>MKYILVTGGVISGIGKGIIASSVGTILKSCGLHVTSIKIDPYINIDAGTFSPYEHGEVFVLDDGGEVDLDLGNYERFLDIRLTKDNNLTTGKIYQYVINKERKGDYLGKTVQVVPHITDAIQEWVMRQALIPVDEDGLEPQVCVIELGGTVGDIESMPFIEAFRQFQFKVKRENFCNIHVSLVPQPSSTGEQKTKPTQNSVRELRGLGLSPDLVVCRCSNPLDTSVKEKISMFCHVEPEQVICVHDVSSIYRVPLLLEEQGVVDYFLRRLDLPIERQPRKMLMKWKEMADRYDRLLETCSIALVGKYTKFSDSYASVIKALEHSALAINHKLEIKYIDSADLEPITSQEEPVRYHEAWQKLCSAHGVLVPGGFGVRGTEGKIQAIAWARNQK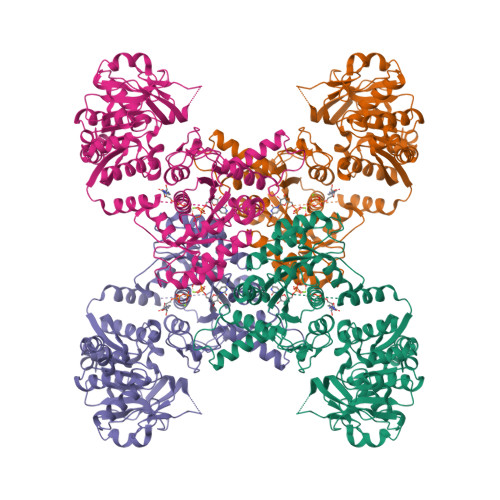KPFLGVCLGMQLAVVEFSRNVLGWQDANSTEFDPTTSHPVVVDMPEHNPGQMGGTMRLGKRRTLFQTKNSVMRKLYGDADYLEERHRHRFEVNPVWKKCLEEQGLKFVGQDVEGERMEIVELEDHPFFVGVQYHPEFLSRPIKPSPPYFGLLLASVGRLSHYLQKGCRLSPRDTYSDRSGSSSPDSEITELKFPSINHD[4x]> GSSLSRTQIVNWLTRCGDIFSTESEYLTGLDREIGDADHGLNMNRGFSKVVEKLPAIADKDIGFILKNT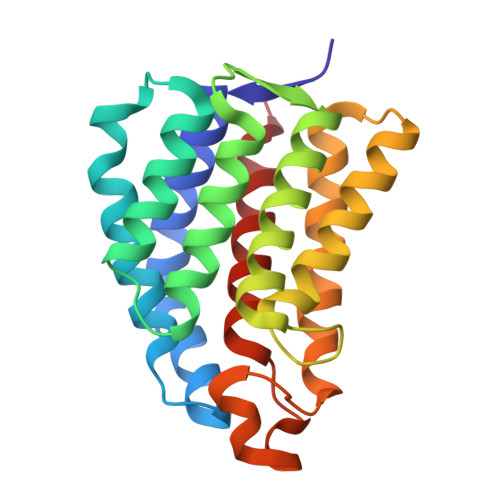GMTLLSSVGGASGPLFGTFFIRAAQATQARQSLTLEELYQMFRDGADGVISRGKAEPGDKTMCDVWVPVVESLRQSSEQNLSVPVALEAASSIAESAAQSTITMQARKGRASYLGERSIGHQDPGATSVMFMMQMLALAAKE> MSVTIDHTTENAAPAQAPVSDRAWALFRALDGKGLVPDGYVEGWKKTFEEDFSPRRGAELVARAWTDPEFRQLLLTDGTAAVAQYGYLGPQGEYIVAVEDTPTLKNVIVCSLCSCTAWPILGLPPTWYKSFEYRARVVREPRKVLSEMGTEIASDIEIRVYDTTAETRYMVLPQRPAGTEGWSQEQLQEIVTKDCLIGVAIPQVPTV;> MDGVHDLAG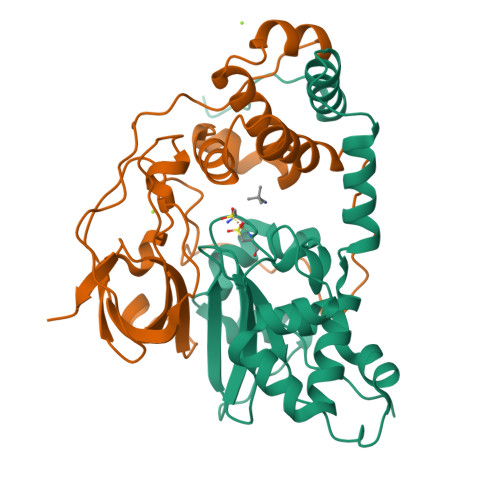VQGFGKVPHTVNADIGPTFHAEWEHLPYSLMFAGVAELGAFSVDEVRYVVERMEPRHYMMTPFYERYVIGVATLMVEKGILTQDELESLAGGPFPLSRPSESEGRPAPVETTTFEVGQRVRVRDEYVPGHIRMPAYCRGRVGTISHRTTEKWPFPDAIGHGRNDAGEEPTYHVKFAAEELFGSDTDGGSVVVDLFEGYLEPAA>[3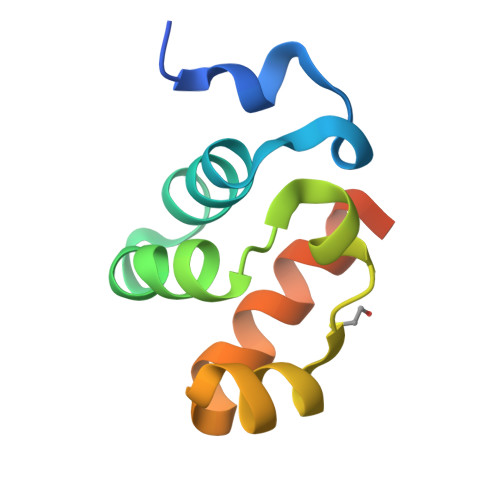x]MEKTRANSHLRSQPIDWTIEEVIQYIESNDNSLAVHGDLFRKHEIDGKALLRLNSEMMMKYMGLKLGPALKICNLVNKVNGRDHHHHHH> GSELQPPEASIAVVSIPRQLPGSHSEAGVQGLSAGDDSELGSHCVAQTGLELLASGDPLPSASQNAEMIETGSDCVTQAGLQLLASSDPPALASKNAEVTGTMSQDTEVDMKEVELNELEPEKQPMNAASGAAMSLAGAEKNGLVKIKVAEDEAEAAAAAKFTGLSKEELLKVAGSPGWVRTRWALLLLFWLGWLGMLAGAVVIIVRAPRCRELPAQKWWHTGALYRIGDLQAFQGHGAGNLAGLKGRLDYLSSLKVKGLVLGPIHKNQKDDVAQTDLLQ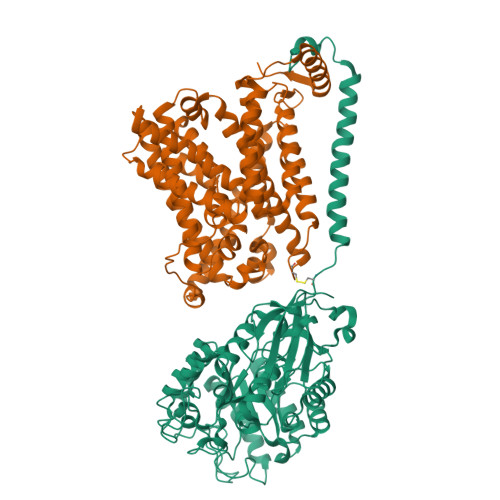IDPNFGSKEDFDSLLQSAKKKSIRVILDLTPNYRGENSWFSTQVDTVATKVKDALEFWLQAGVDGFQVRDIENLKDASSFLAEWQNITKGFSEDRLLIAGTNSSDLQQILSLLESNKDLLLTSSYLSDSGSTGEHTKSLVTQYLNATGNRWCSWSLSQARLLTSFLPAQLLRLYQLMLFTLPGTPVFSYGDEIGLDAAALPGQPMEAPVMLWDESSFPDIPGAVSANMTVKGQSEDPGSLLSLFRRLSDQRSKERSLLHGDFHAFSAGPGLFSYIRHWDQNERFLVVLNFGDVGLSAGLQASDLPASASLPAKADLLLSTQPGREEGSPLELERLKLEPHEGLLLRFPYAA;> MVRKPVVSTISKGGYLQGNVNGRLPSLGSKEPPGQEKVQLKREITLLDGVSLIVGTIIGAGIFVSPKGVLKNTGSVGLSLVIWAVCGVLSLFGALCYAELGTTIPKSGGAYLYILETFGPLPAFLRGWNELLIIRPASTAVISLAFGNYILEPFFPTCEPPELAIKLLAAVGILLLTVLNSLSVKWSARVQDFFTAAKLLALLIIIVPGVVQLIKGQTQNFKDAFEGSDPSIGGLPLAFYSGLYAYVGWDYLNFVTEEVKNPEKNIPLAIVISMPIVTVAYVLTNVAYFTTLSPEELLLSNAVAVTFGERLLGNFSWAVPIFVALSCFGSLNGSLFAMSRLFYVAAREGHLPKILSMIHVRRHTPLPALIVSGPLTAIMLFLGDLFSLINFMSFGTWLFYGLVVAGLIYLRYKKPDLHRPIKVPLFIPILFLLTCLFLVAVSLYSDPVNCGIGFVIILTGVPVYFLFVYWDKKPKWFRRISEKITRHLQLLLEVVPEEDKLDYKDDDDK6-bromanyl-3-chloranyl-quinolin-8-ol 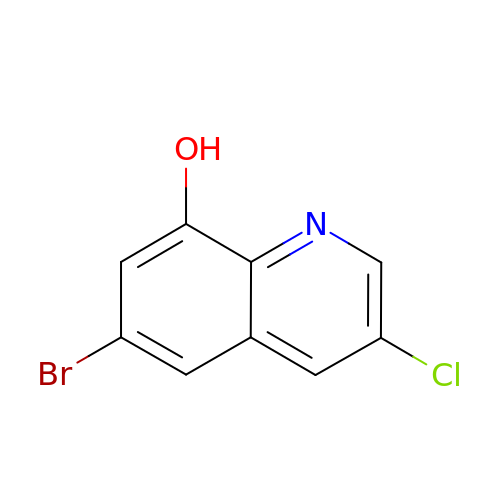| C9 H5 Br Cl N O | IYXNDLZQIYAJTB-UHFFFAOYSA-N> MSLDRVDWPHATFSTPVKRIFDTQTTLDFQSSLAIHRIKYHLHKYTTLISHCSDPDPHATASS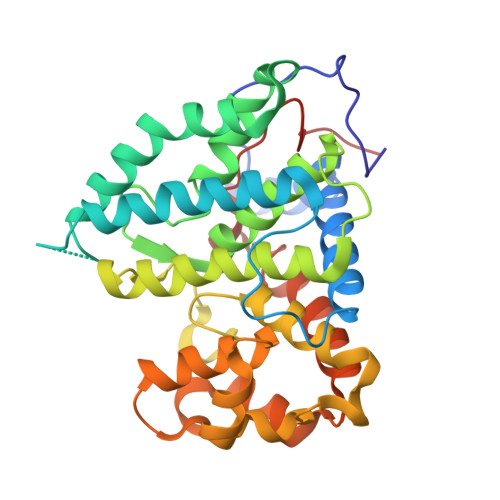IAMVNGLMGVLDKLAHLIDETPPLPGPRRYGNLACREWHHKLDERLPQWLQEMLPSEYHEVVPELQYYLGNSFGSSTRLDYGTGHELSFMATVAALDMLGMFPHMRGADVFLLFNKYYTIMRRLILTYTLEPAGSHGVWGLDDHFHLVYILGSSQWQLLDAQAPLQPREILDKSLVREYKDTNFYCQGINFINEVKMGPFEEHSPILYDIAVTVPRWSKVCKGLLKMYSVEVLKKFPVVQHFWFGTGFFPWVNIHHHHHH>[2x]GASNEVLVLRGTLEGHNGWVTSLATSAGQPNLLLSASRDKTLISWKLTGDDQKFGVPVRSFKGHSHIVQDCTLTADGAYALSASWDKTLRLWDVATGETYQRFVGHKSDVMSVDIDKKASMIISGSRDKTIKVWTIKGQCLATLLGHNDWVSQVRVVPNEKADD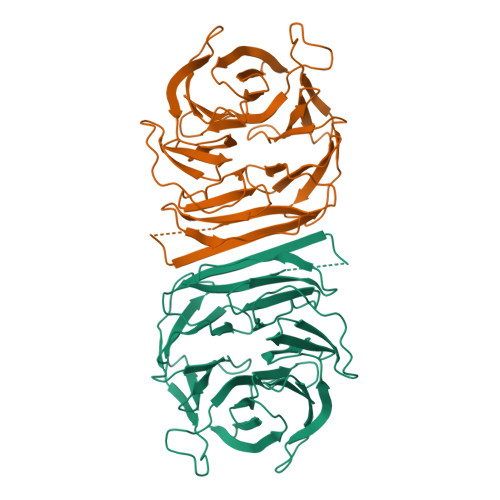DSVTIISAGNDKMVKAWNLNQFQIEADFIGHNSNINTLTASPDGTLIASAGKDGEIMLWNLAAKKAMYTLSAQDEVFSLAFSPNRYWLAAATATGIKVFSLDPQYLVDDLRPEFAGYSKAAEPHAVSLAWSADGQTLFAGYTDNVIRVWQVMTAN>[2x]MGSDKIHHHHHHMNNTIPRWRGFNLLEAFSIKSTGNFKEEDFLWMAQWDFNFVRIPMCHLLWSDRGNPFIIREDFFEKIDRVIFWGEKYGIHICISLHRAPGYSVNK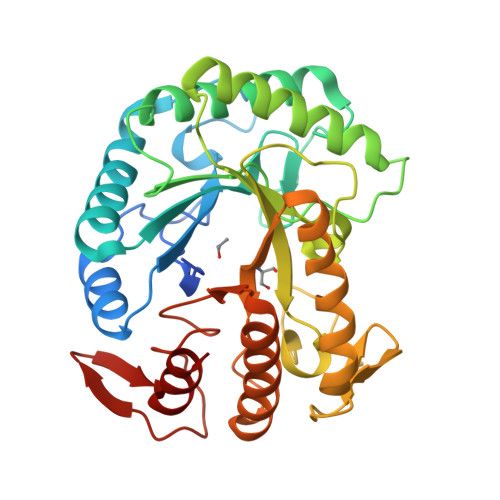EVEEKTNLWKDETAQEAFIHHWSFIARRYKGISSTHLSFNLINEPPFPDPQIMSVEDHNSLIKRTITEIRKIDPERLIIIDGLGYGNIPVDDLTIENTVQSCRGYIPFSVTHYKAEWVDSKDFPVPEWPNGWHFGEYWNREKLLEHYLTWIKLRQKGIEVFCGEMGAYNKTPHDVVLKWLEDLLEIFKTLNIGFALWNFRGPFGILDSERKDVEYEEWYGHKLDRKMLELLRKY Our comparative bioinformatics studies suggest that among those reported as glycosyltransferases are also pseudo-glycosyltransferases (such as VldE, EC 2.x.x.x), which do not recognize sugars as substrates but rather catalyze the formation of non-glycosidic C-N bonds in the biosynthesis of C7N-aminocyclitol-containing natural products such as acarbose and validamycin A. Validoxylamine A is generated through the dephosphorylation of validoxylamine A 7′-phosphate by VldH while validoxylamine A 7′-phosphate (VDO) results from a condensation of GDP-valienol and validamine 7-phosphate (both are pseudo-sugars) by the pseudo-glycosyltransferase, VldE. Similar to OtsA, VldE is comprised of two Rossman β/α/β domains which are oriented in a GT-B configuration. As was described in a recent crystallographic study of ValL, a VldE homolog from S. hygroscopicus subsp. jinganggensis, VldE is a homodimer.

Within the VldE•GDP•TRE structure, six monomers were modeled within the asymmetric unit (ASU). Represented within the six monomers were three differing conformations of the N-terminal Rossman-like domain (two monomers per conformation). The monomers of the first conformation contained both GDP and trehalose, and this first conformer was found to also have an “open” catalytic site with similar global conformation to the VldE•GDP•VDO complex (RMSD Cα = 0.705 Å). The sugar moiety of trehalose within donor cyclitol binding site makes interactions with the backbone amides of residues Gly384, Gln385, Asn386, and Leu387 as well with the side-chains of Asp383 and His182. However, the sugar moiety of trehalose occupying the acceptor cyclitol binding site makes only a single hydrogen bond with Arg290 in our study. A superimposition of trehalose and VDO within the VldE catalytic site shows that trehalose does not assume a binding pose comparable to VDO. Indicatively, Arg326 and Asn325 swing out of the catalytic site within our trehalose bound structure. The second and third conformers have only GDP within the catalytic site and both of these conformers share a dramatic shift in residues 11–50 which result in the “closing” of the catalytic site. Resultantly, Gly33, Gly34, and Thr35 move 10.9 Å towards the catalytic center, and within 4 Å of the ligand atoms. Therefore, the closing of the VldE catalytic site is more likely to work at least partially through a more dynamic, equilibrium based mechanism.

>MTGSEIFLASKRAAITYDTDPATGEPRAWLAPGGTGNVVAEQAGVLNISWIASADSEDDRRASALNPDGVTMELHSGREILVRLIRHDPAVFRNVQNFMTANLMWAANNYGWDRWTQPSFGSDAREGWADFGRFTRDFADAILKSSAQSADPVYLVHDYQLVGVPALLREQRPDAPILLFVHIPWPSADYWRILPKEIRTGILHGMLPATTIGFFADRWCRNFLESVADLLPDARIDREAMTVEWRGHRTRLRTMPLGYSPLTLDGRNPQLPEGIEEWADGHRLVVHSGRTDPIKNAERAVRAFVLAARGGGLEKTRMLVRMNPNRLYVPANADYVHRVETAVAEANAELGSDTVRIDNDNDVNHTIACFRRADLLIFNSTVDGQNLSTFEAPLVNERDADVILSETCGAAEVLGEYCRSVNPFDLVEQAEAISAALAAGPRQRAEAAARRRDAARPWTLEAWVQAQLDGLAADHAARTATAERFDTAPAVSTRADL[6x]> MEKETTQGTTYYVSSSKGDDSNDGTSESKPFKTLEKINKLTLKPGDQVLLEKGSVFNDQYLHLKGSGSAEAPIKVSTYGEGNRPQILTNGQGLWELNYGKHLDNTNHKWHGTVSSSILLKDVEYIEIEGLEITNDRGTKNDPEGDKAYNDADCMDRTGVAGVAKDKGTLDHIVLDDLYIHDVDGNVYNKHMTNGGIYFIVEKPTDENKTGIAKYDDVQIKNCQLDTVNRWGIAVGYTYNWDKFQTAELSDEVMEKYGATNVVIENNYLNNVGGDAITTMYADEPLIQYNVSENS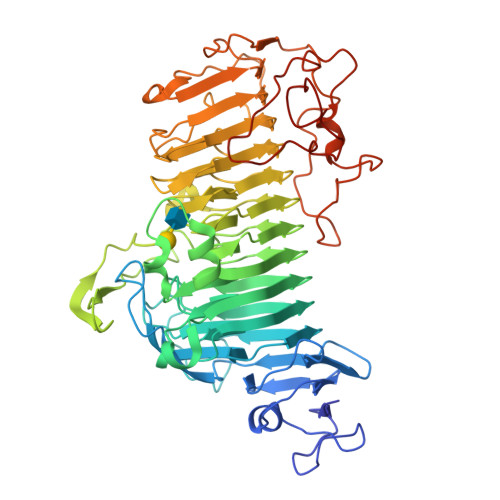SKQINKTDYSKPQPVLDKVTGEPTGQYQGVGAGRVAAGIWPWKCKNAVFQYNECFRTLNASNGNGDGQPWDADYGDGTNYQYNYSHGNTASTIMFCGYQSVNNTFRYNISQNEDMGPLDPAGNAGNTQVYNNTFYIKEGLNNIWHTSHGNAGPINLENNIFYFAGETPATVENWNPNGNKTYSNNLFYNVSTYPEDANAVKVDAGTKVTENAGSGPSTVADDKQARRHEDPSAETVFDGYKLVQNSPAINAGKIIVDNNGYKVEKDFFGNKVSGIPDIGAHEAAALEHHHHHH4-[4-(3-chlorophenyl)piperazin-1-yl]-4-oxobutane-1-thiol | C14 H19 Cl N2 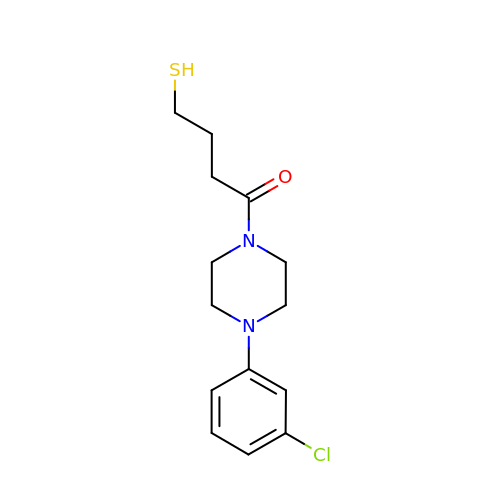O S | ZRDBMFDEDKLQCF-UHFFFAOYSA-N> QQGNPNLSSPQPILDTIYKLLSEQEQTLVQMIHEQSLLLNRLPPTLDENSLAPLKSLSQKQITLSGQMNTEMSALDATKKGMILEPTDLAKLFALKQDLQIQFKQLSLLHNEIQSILNPQHSAPKPNVALVLKSQPFPVVISKGKQLGENQLVVLVLTGARSNFHINGPVKATMICDSHPTNKNNPTTPLEMDSQPIYPATLTAHFPLKFLAGTRKCSVNLKFGVNIRDLDNVTTTVESDASNPFVVITNECQWEGSAGVLLKKDAFDGQLEI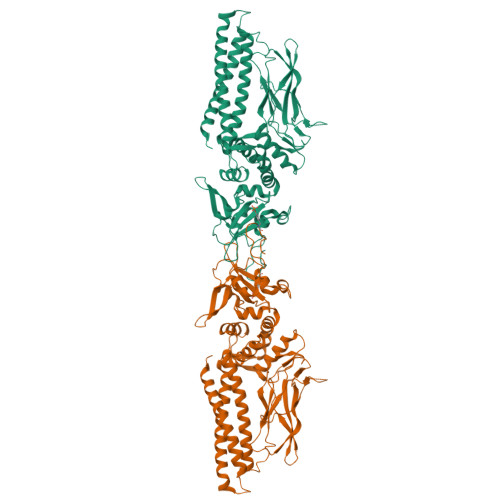TWAQFINTLQRHFLIATKQDPVRPKRPLSSYDLKYIQTHFFGNRSIIHQQDFDKFWVWFGKSMQTLRYQRHISTLWQEGIIYGYMGRQEVNDALQNQDPGTFIIRFSERNPGQFGIAYIGVEMPARIKHYLVQPNDTAAAKKTFPDFLSEHSQFVNLLQWTKDTNGAPRFLKLHKDTALGSFAPKRTAPVPVGGYEPLNS>[3x]MFKIVYPNAKDFFSFINSITNVTDSIILNFTEDGIFSRHLTEDKVLMAIMRIPKDVLSEYSIDSPTSVKLDVSSVKKILSKASSKKATIELTETDSGLKIIIRDEKSGAKSTIYIKAEKGQVEQLTEPKVNLAVNFTTDESVLNVIAADVTLVGEEMRISTEEDKIKIEAGEEGKRYVAFLMKDKPLKELSIDTSASSSYSAEMFKDAVKGLRGFSAPTMVSFGENLPMKIDVEA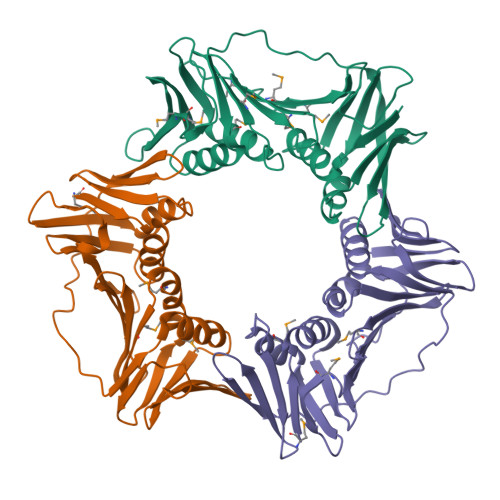VSGGHMIFWIAPRLLEHHHHHH;>[3x]MKAKVIDAVSFSYILRTVGDFLSEANFIVTKEGIRVSGIDPSRVVFLDIFLPSSYFEGFEVSQEKEIIGFKLEDVNDILKRVLKDDTLILSSNESKLTLTFDGEFTRSFELPLIQVESTQPPSVNLEFPFKAQLLTITFADIIDELSDLGEVLNIHSKENKLYFEVIGDLSTAKVELSTDNGTLLEASGADVSSSYGMEYVANTTKMRRASDSMELYFGSQIPLKLRFKLPQEGYGDFYIAPRAD;>MKVVYDDVRVLKDIIQALARLVDEAVLKFKQDSVELVALDRAHISLISVNLPREMFKEYDVNDEFKFGFNTQYLMKILKVAKRKEAIEIASESPDSVIINIIGSTNREFNVRNLEVSEQEIPEINLQFDISATISSDGFKSAISEVSTVTDNVVVEGHEDRILIKAEGESEVEVEFSKDTGGLQDLEFSKESKNSYSAEYLDDVLSLTKLSDYVKISFGNQKPLQLFFNMEGGGKVTYLLAPKVLEHHHHHH[3x]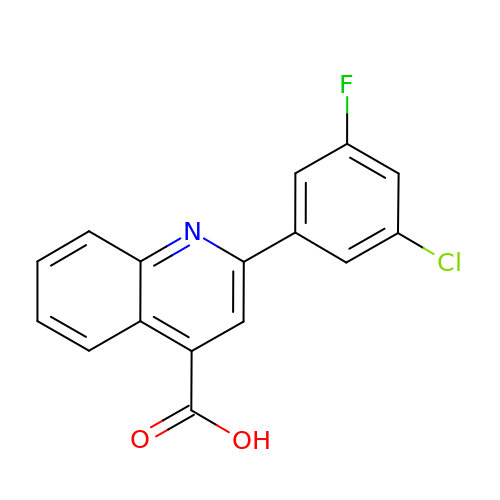2-(3-chloranyl-5-fluoranyl-phenyl)quinoline-4-carboxylic acid | C16 H9 Cl F N O2 | NIKQCFUMVUWEJP-UHFFFAOYSA-N>[2x]CDSYLDIRPVGSVIPQTAEEYRALLARAYLNVPNDRGLACLRSDEMLVNDNEYDRNSYGDIERWNDVSPFPGTSQFTWSNFYNVLFIANQVIESQKEITEGTPEVVNQLVGEAHLLRAYLHFVLVNLHGQPYTKSGALNSKSIPLKLDTDLEKTLGRNTVEEVYTSILSDIEHARELINKEKWETVFSYRFNVLSVDALQSRVSLYMGAWPKCLESAEAVLAKKSVLVDMNETPLALPNHFESVESITALEQVMGSSVNNAVWVPATFLALYQEGDKRLAAYFAAPDENGNRKSSKGGKREFSCTFRVGELYLNAAEAAANMDKLPHARMRLLELMRKRYTPEAYAKKENAVNVMDKNALISEILNERARELAFEGHRWFDLRRTTRPRMVKVLQGKTYILEQDDPRYTIPIPRDAIAANPGL;>[2x]DAVVVTGYQTVERRKLTAAVGKLNISDETIGAVKSIDQALAGQIAGLSVTSTSGAPGAPAKIRIRGTSSLNGTQDPLWVLDGIPLEGTDVPQSNVLNDVSNIQQSSIAGLNPADIENITVLKDAAATAIYGARAANGVIVITTKKGKVGKPVINFSSKFTYM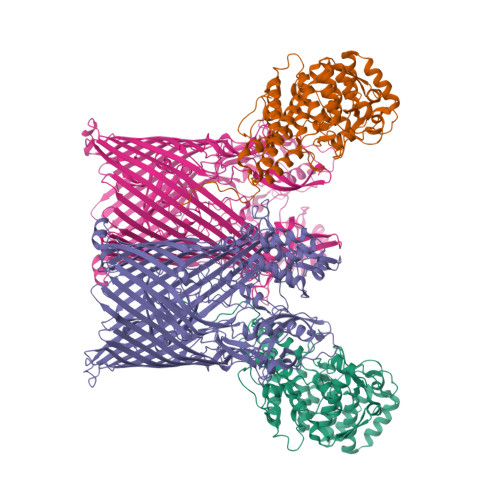PTLSTNRLNMLNSQEKVDLELELLRSNFAYGDNKGGVSKIISGYGLTDAYKKGGWSALTPEAQTDISRLRNTETDWGDILFRDAFNQEYSLSLSGGNERVTYYTSIGYYQENGNVKGVGLDRLNIVAKTSYKVNRMLKFGVSLFVNRRNNKTYLTDTYGLVNPVYYSRKANPYYQPFDANGNYVYDFDVQNNSDTDLGFNIFEERKNTSNEETINALSSIFDAELRFNDKLKFTTQLGLQLDKASKEQIADKESFSMRIIRKNSKYWDSASQSNKYFIPDGGVHKAYENTNSQITWKAMGEYRDSFNDIHELEVMVGTELRKTWYETLFSAGYGFDRQTLTTKPVVFPDEDRARQFPLHQKTYKENAYVSFFSTASYSLMNRYTFGGSIRFDGSDLFGVDKKYRYLPLYSVSGLWRLSNEPFMQGTRKWMDNLAFRVSYGIQGNIDKNTSPFLLGKYIVDNILPGGSEHMIDINSAPNKKLRWEKTQSVNVGLDFSVLNQALNLSVDYYYRKGTDLIGKQMLPLETGFVSTNINWASMVNKGVEVSLSTRNVATKNFSWYTNLNFAYNNNKVLREAIPEAQTIPGREGYPVDAIFAIKTAGLDEEGYPLFYDKEGKKVTLKELYRLQDPFGLGFTVNSDVTPAEERSFYSYIGSQDTPYTGGLINTFSYKNWELTANLSFNLGGYVRTTPSYNFINFDRGQNVNSDILDRWTPENTDGRLPALITSEKRADEYYWYDQKSEIYKNLDIWVKKLNYFRLQNLRLGYRLPEKMTKSLGMGSASVAIEGRNLLVFGSSYKNFLDPESMYNPYAPPIPKSITFSLNLNF4-HYDROXYPHENYLACETATE | C8 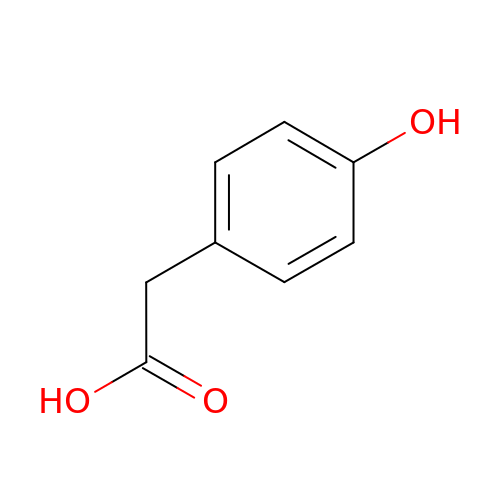H8 O3 | XQXPVVBIMDBYFF-UHFFFAOYSA-N>MDKNWFSTPQEIREGIKYLSAHFYPASIMDRWKILKKLSFEKAKIIANYSLQQVIEEIEHFDFFNEYFKEDPLTTVRLPPSYIKLFDGLVEDFQSSRWRENIATRFHMITEGVLATVGLKILNETSRKYNLLKFNEGIKRIIEDEARHVS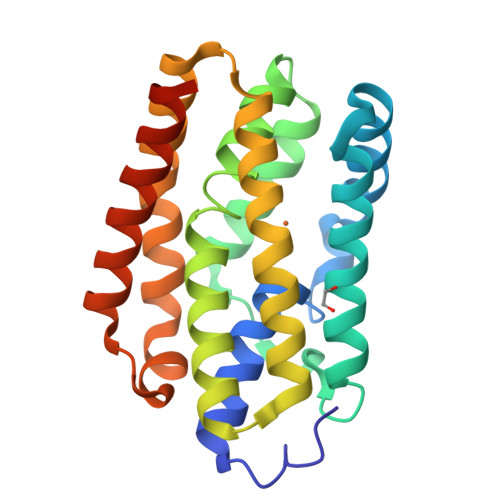FGLSLIEDKEYAVKRVEELFPLAVQIVKEGKDKIEPLGYSIQELVNLMEELKKARINKILGSGSHHHHHH[2x]> MRGSHHHHHHGLVPRGSMDNVIGLEIIEVVEQAAIASARWMGKGDKNMADQAAVDAMRNRMNQIHMRGRIVIGEGERDEAPMLYIGEEVGICTRPDAAQ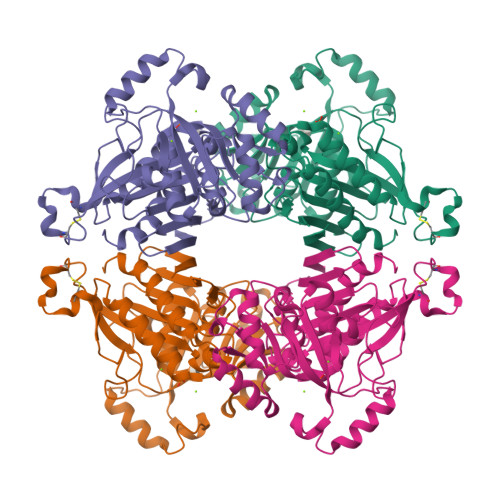YCNPEELIEIDIAVDPCEGTNLCAYGQPGSMAVLAISEKGGLFAAPDFYMKKLAAPPAAKGKVDIRNSATENLKILSECLDRAIDELVVVVMKRDRHNDLIQEIRDAGARVQLISDGDVSAALACAFSGTNIHALMGIGAAPEGVISAAAMRALGGHFQGQLVYDPAVVMTKEWANRTREGNLEELKKAGITDPDKVYEAEELASGETVLFAACGITPGMLMKGVRFFKGGARTQSLVISTQSKTARFVDTIHMFDQQLKSLQLY> GSHMVPISFVFNRFPRMVRDLAKKMNKEVNFIMRGEDTELDRTFVEEIGEPLLHLLRNAIDHGIEPKEERIAKGKPPIGTLILSARHEGNNVVIEVEDDGRGIDKEKIIRKAIEKGLIDESKAATLSDQEILNFLFVPGFSTKEKVSEVSGRGVGMDVVKNVVESLNGSISIESEKDKGTKVTIRLPLTLAIIQALLVKVNNLVYAIPIANIDTILSISKEDIQRVQDRDVIVIRGEVI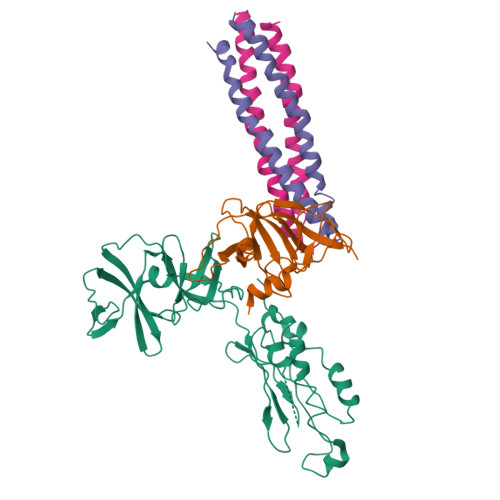PVYRLWEVLQIEHKEELEEMEAVIVRVGNRKYGIVVDDLLGQDDIVIKSLGKVFSEVKEFSGAAILGDGSIALIINVSGIV;> KEFEVLSFEIDEQALAFDVDNIEMVIEKSDITPVPKSRHFVEGVINLRGRIIPVVNLAKILGISFDEQKMKSIIVARTKDVEVGFLVDRVLGVLRITENQLDLTNVSDKFGKKSKGLVKTDGRLIIYLDIDKIIEEITV;>[2x]SQIGETLENIRSIEKLIQNIMRIARETNILALNATIEAARAGEAGKGFMIVANEVQNLSNETNEVTKQIVEKAREILESSQRSLE>[2x]MVALSAEGSSGGSRGGSPKAEAASVPSWPQILG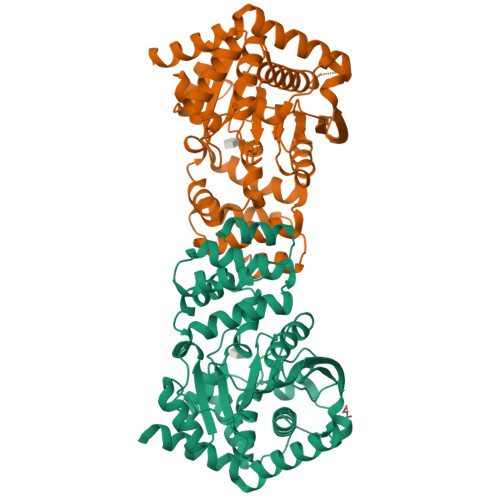RLTDNRDLARGQAAWAMDQIMTGNARPAQIAAFAVAMTMKAPTADEVGELAGVMLSHAHPLPADTVPDDAVDVVGTGGDGVNTVNLSTMAAIVVAAAGVPVVKHGNRAASSLSGGADTLEALGVRIDLGPDLVARSLAEVGIGFCFAPRFHPSYRHAAAVRREIGVPTVFNLLGPLTNPARPRAGLIGCAFADLAEVMAGVFAARRSSVLVVHGDDGLDELTTTTTSTIWRVAAGSVDKLTFDPAGFGFARAQLDQLAGGDAQANAAAVRAVLGGARGPVRDAVVLNAAGAIVAHAGLSSRAEWLPAWEEGLRRASAAIDTGAAEQLLARWVRFGRQILEHHHHHH>[3x]MRRTTKETDIIVEIGKKGEIKTNDLILDHMLTAFAFYLGKDMRITATYDLRHHLWEDIGITLGEALRENLPEKFTRFGNAIMPMDDALV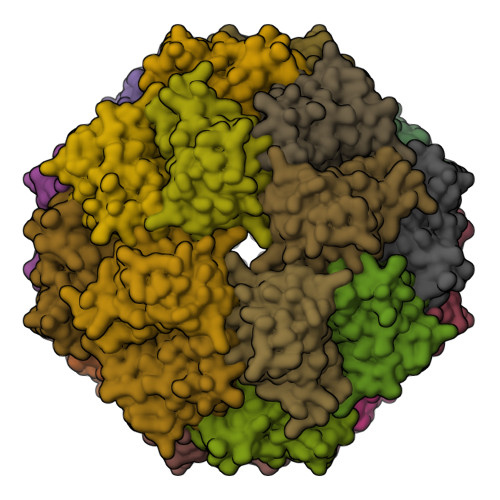LVSVDISNRPYANVDVNIKDAEEGFAVSLLKEFVWGLARGLRATIHIKQLSGENAHHIVEAAFKGLGMALRVATKESERVESTKGVL> MKKHHHHHHGSLVPRGSKLEINKFNYNDPIDGINVITMRPPRHSDKINKGKGPFKAFQVIKNIWIVPERYNFTNNTNDLNIPSEPIMEADAIYNPNY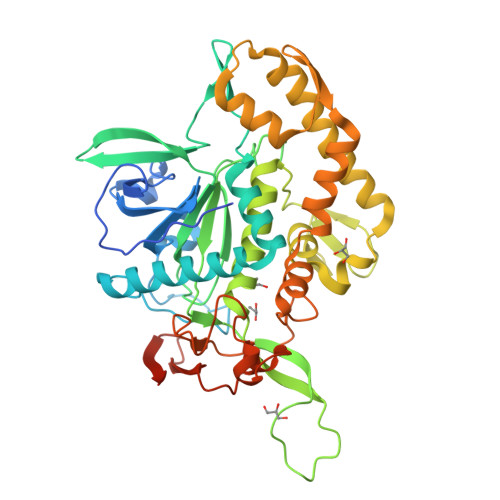LNTPSEKDEFLQGVIKVLERIKSKPEGEKLLELISSSIPLPLVSNGALTLSDNETIAYQENNNIVSNLQANLVIYGPGPDIANNATYGLYSTPISNGEGTLSEVSFSPFYLKPFDESYGNYRSLVNIVNKFVKREFAPDPASTLMHELVHVTHNLYGISNRNFYYNFDTGKIETSRQQNSLIFEELLTFGGIDSKAISSLIIKKIIETAKNNYTTLISERLNTVTVENDLLKYIKNKIPVQGRLGNFKLDTAEFEKKLNTILFVLNESNLAQRFSILVRKHYLKERPIDPIYVNILDDNSYSTLEGFNISSQGSNDFQGQLLESSYFEKIESNALRAFIKICPRNGLLYNAIYRNSKNYLN> GMRVGVLGAKGKVGATMVRAVAAADDLTLSAELDAGDPLSLLTDGNTEV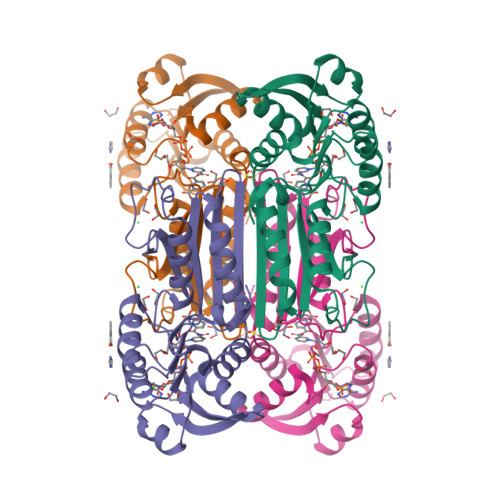VIDFTHPDVVMGNLEFLIDNGIHAVVGTTGFTAERFQQVESWLVAKPNTSVLIAPNFAIGAVLSMHFAKQAARFFDSAEVIELHHPHKADAPSGTAARTAKLIAEARKGLPPNPDATSTSLPGARGADVDGIPVHAVRLAGLVAHQEVLFGTEGETLTIRHDSLDRTSFVPGVLLAVRRIAERPGLTVGLEPLLDL N-Acyl homoserine lactonases (AHL-lactonases) have important functions in decreasing pathogenicity by degrading AHLs. Unlike most AHL-lactonases, AidH is proposed to be a member of the α/β-hydrolase fold family. AidH contains a substrate-binding tunnel between the core domain and the cap domain. Taken together, the present results reveal the catalytic mechanism of the metal-independent AHL-lactonase, which is a typical acid–base covalent catalysis.

The crystal structure of AidH was determined at 1.29 Å resolution using single-wavelength anomalous dispersion (SAD) phasing. The crystal has the symmetry of space group P21 and contains two molecules per asymmetric unit. Size-exclusion chromatography and analytical ultracentrifugation data for AidH indicate that it is monomeric in solution. Therefore, the functional unit of the enzyme is a monomer and the dimeric organization on crystallization is likely to be an artifact of the crystal packing. The α/β-hydrolase fold core domain consists of an eight-stranded mostly parallel β-sheet (only the second β-strand, β2, is antiparallel to the rest) surrounded by seven α-­helices. The cap domain composed of five α-helices is inserted between strands β6 and α4 of the core domain. The whole active site is covered by the cap domain. (i) The structure of AidH shows that it possesses a conserved catalytic triad (Ser102, His248 and Glu219) and a recognizable substrate-binding tunnel. A hydrogen-bond network connects Ser102 to Glu219 via His248. No metal ion is bound in the active site, which is different from other AHL-lactonases, which have a dual Lewis acid catalysis mechanism.

>[2x]MTINYHELETSHGRIAVRESEGEGAPLLMIHGNSSSGAIFAPQLEGEIGKKWRVIAPDLPGHGKSTDAIDPDRSYSMEGYADAMTEVMQQLGIADAVVFGWSLGGHIGIEMIARYPEMRGLMITGTPPVAREEVGQGFKSGPDMALAGQEIFSERDVESYARSTCGEPFEASLLDIVARTDGRARRIMFEKFGSGTGGNQRDIVAEAQLPIAVVNGRDEPFVELDFVSKVKFGNLWEGKTHVIDNAGHAPFREAPAEFDAYLARFIRDCTQLEHHHHHH> MGSSHHHHHHSSGPQQGLRKGDIKIKIVSGTASSFQSGSNIEKSFDGDYSTLYHSSWSNGASNYFPITLTYNFETVTDVDYLIYHPRNNGNNGRFKETEIQYSADGHT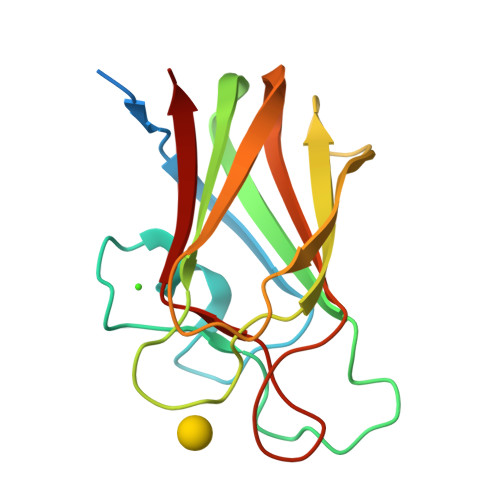FTKLIDKDFQGSATAGKVTFDQTIQAKSFRFIVKSGSGDGQGFASCAEMEFFAK>AAPDEITTAWPVNVGPLNPHLYTPNQMFAQSMVYEPLVKYQADGSVIPWLAKSWTHSEDGKTWTFTLRDDVKFSNGEPFDAEAAAENFRAVLDNRQRHAWLELANQIVDVKALSKTELQITLKSAYYPFLQELALPRPFRFIAPSQFKNHETMNGIKAPIGTGPWILQESKLNQYDVFVRNENYWGEKPAIKKITFNVIPDPTTRAVAFETGDIDLLYGNEGLLPLDTFARFSQNPAYHTQLSQPIETVMLALNTAKAPTNELAVREALNYAVNKKSLIDNALYGTQQVADTLFAPSVPYANLGLKPSQYDPQKAKALLEKAGWTLPAGKDIREKNGQPLRIELSFIGTDALSKSMAEIIQADMRQIGADVSLIGEEESSIYARQRDGRFGMIFHRTWGAPYDPHAFLSSMRVPSHADFQAQQGLADKPLIDKEIGEVLAT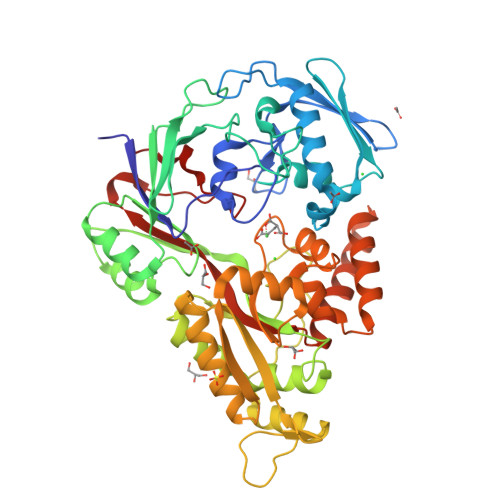HDETQRQALYRDILTRLHDEAVYLPISYISMMVVSKPELGNIPYAPIATEIPFEQIKPVKP[3x]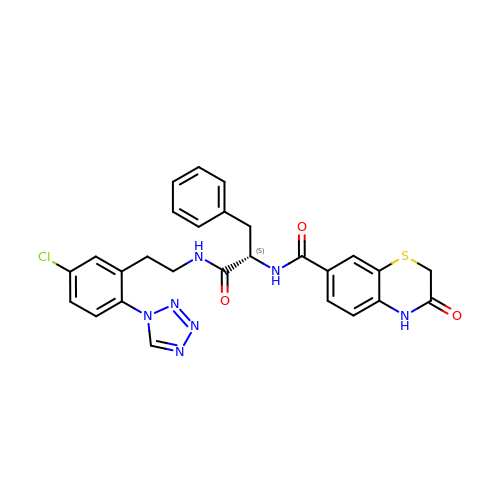N-[(2S)-1-({2-[5-chloro-2-(1H-tetrazol-1-yl)phenyl]ethyl}amino)-1-oxo-3-phenylpropan-2-yl]-3-oxo-3,4-dihydro-2H-1,4-benzothiazine-7-carboxamide | C27 H24 Cl N7 O3 S | IAXDWTLDVZYTHX-QFIPXVFZSA-N> MALSKLNHLYMAVVADHSKRPHHHGQLDGVEAVQ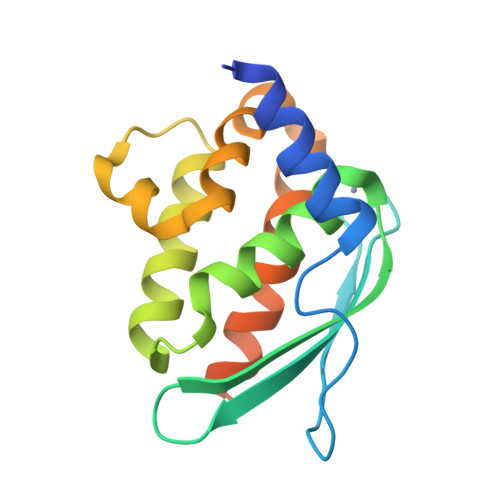LNNPTCGDVISLTVKFDEDKIEDIAFAGNGCTISTASSSMMTDAVIGKSKEEALALADIFSEMVQGQENPAQKELGEAELLAGVAKFPQRIKCSTLAWNALKEAIKRSANAQHLTDQNVKEGKNV10-[3-(4-METHYL-PIPERAZIN-1-YL)-PROPYL]-2-TRIFLUOROMETHYL-10H-PHENOTHIAZINE | C21 H24 F3 N3 S | 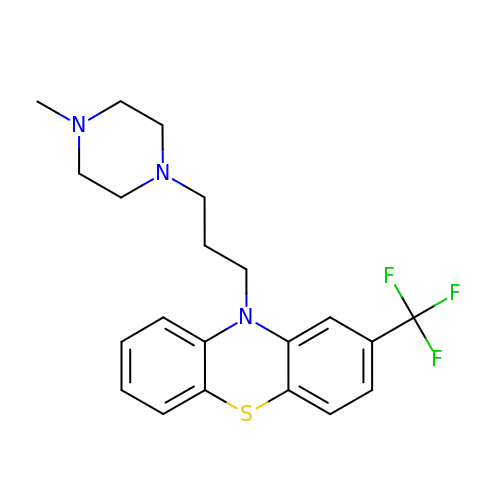ZEWQUBUPAILYHI-UHFFFAOYSA-N> GDRVADVIESSIGDSVSRALTHALPAPTGQNTQVSSHRLDTGKVPALQAAEIGASSNASDESMIETRCVLNSHSTAETTLDSFFSRAGLVGEIDLPLEGTSVKRGTSVGMKPSPRPTNPNGYANWDIDITGYAQMRRKVELFTYMRFDAEFTFVACTPTGEVVPQLLQYMFVPPGAPKPDSRESLAWQTATNPSVFVKLSDPPAQVSVPFMSPASAYQWFYDGYPTFGEHKQEKDLEYGACPNN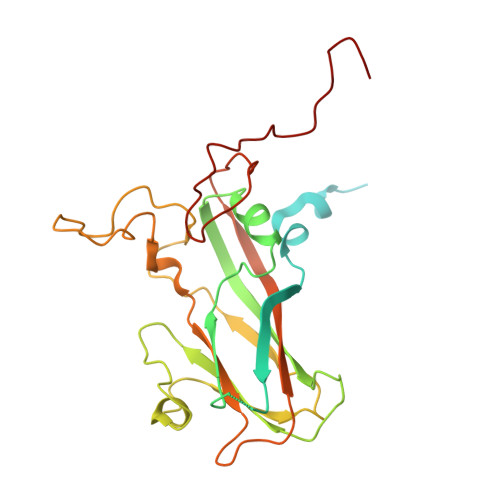MMGTFSVRTVGTSKSKYPLVVRIYMRMKHVRAWIPRPMRNQNYLFKANPNYAGNSIKPTGASRTAITTL>[2x]MGSSHHHHHHQNVSLQPPPQQLIVQNKTIDLPAVYQLNGGEEANPHAVKVLKELLSGKQSSKKGMLISIGEKGDKSVRKYSRQIPDHKEGYYLSVNEKEIVLAGNDERGTYYALQTFAQLL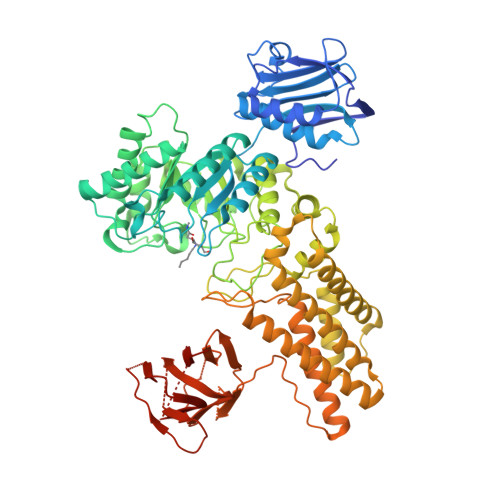KDGKLPEVEIKDYPSVRYRGVVEGFYGTPWSHQARLSQLKFYGKNKMNTYIYGPKDDPYHSAPNWRLPYPDKEAAQLQELVAVANENEVDFVWAIHPGQDIKWNKEDRDLLLAKFEKMYQLGVRSFAVFFDDISGEGTNPQKQAELLNYIDEKFAQVKPDINQLVMCPTEYNKSWSNPNGNYLTTLGDKLNPSIQIMWTGDRVISDITRDGISWINERIKRPAYIWWNFPVSDYVRDHLLLGPVYGNDTTIAKEMSGFVTNPMEHAESSKIAIYSVASYAWNPAKYDTWQTWKDAIRTILPSAAEELECFAMHNSDLGPNGHGYRREESMDIQPAAERFLKAFKEGKNYDKADFETLQYTFERMKESADILLMNTENKPLIVEITPWVHQFKLTAEMGEEVLKMVEGRNESYFLRKYNHVKALQQQMFYIDQTSNQNPYQPGVKTATRVIKPLIDRTFATVVKFFNQKFNAHLDATTDYMPHKMISNVEQIKNLPLQVKANRVLISPANEVVKWAAGNSVEIELDAIYPGENIQINFGKDAPCTWGRLEISTDGKEWKTVDLKQKESRLSAGLQKAPVKFVRFTNVSDEEQQVYLRQFVLTIEKK>EVSQDLFNQFNLFAQYSAAAYCGKNNDAPAGTNITCTGNACPEVEKADATFLYSFEDSGVGDVTGFLALDNTNKLIVLSFRGSRSIENWIGNLNFDLKEINDICSGCRGHDGFTSSWRS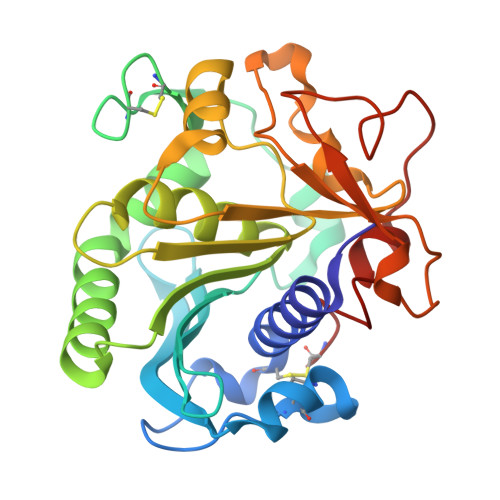VADTLRQKVEDAVREHPDYRVVFTGHSLGGALATVAGADLRGNGYDIDVFSYGAPRVGNRAFAEFLTVQTGGTLYRITHTNDIVPRLPPREFGYSHSSPEYWIKSGTLVPVTRNDIVKIEGIDATGGNNQPNIPDIPAHLWYFGLIGTCL[4x]> PDVVLVNGGEPPNPLIPTGTNDSNGGRIIDRLFAGLMSYDAVGKPSLEVAQSIESADNVNYRITVKPGWKFTDGSPVTAHSFVDAWNYGALSTNAQLQQHFFSPIEGFDDVAGAPGDKSRTTMSGLRVVNDLEFTVRLKAPTIDFTLALGHSSFYPLPDSAFRDMAAFGRNPIGNGPYKLADGPAGPAWEHNVRIDLV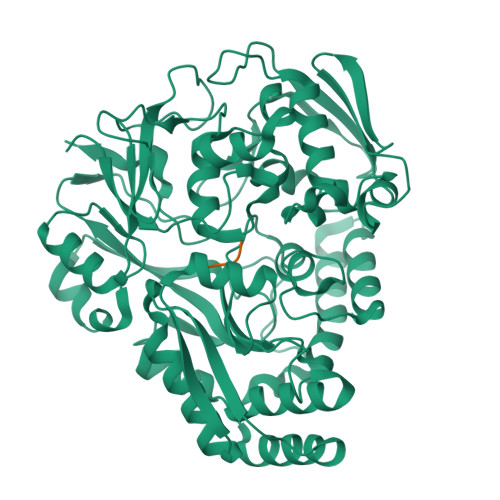PNPDYHGNRKPRNKGLRFEFYANLDTAYADLLSGNLDVLDTIPPSALTVYQRDLGDHATSGPAAINQTLDTPLRLPHFGGEEGRLRRLALSAAINRPQICQQIFAGTRSPARDFTARSLPGFDPNLPGNEVLDYDPQRARRLWAQADAISPWSGRYAIAYNADAGHRDWVDAVANSIKNVLGIDAVAAPQPTFAGFRTQITNRAIDSAFRAGWRGDYPSMIEFLAPLFTAGAGSNDVGYINPEFDAALAAAEAAPTLTESHELVNDAQRILFHDMPVVPLWDYISVVGWSSQVSNVTVTWNGLPDYENIVKA;> VVVA> MPTQKELRDTMSKKLQEAIKHPDPAVVAGRKSAIKRWVGVLQDNFMEHIKYFKGDKLKFLHNVFQDEGCWSGVRLDNAALGQRFTEEKIGGIDNPLRKYEMACSYCVVDKIHPLFQKRFESYRNKFPPGAFDGKTETEFGKYVRNSLLDSIKRKGPVFDFWIDRESGELKKYDAVEGFDSAVKFKWSEGVEYFYNHLKEEDKEKKLTEAILALSRVQSVEKDAPILDFCVNKIVDKDTLLQKLSQKDKGVYSLFVELIESCFFDTVHDLVQCWCYKE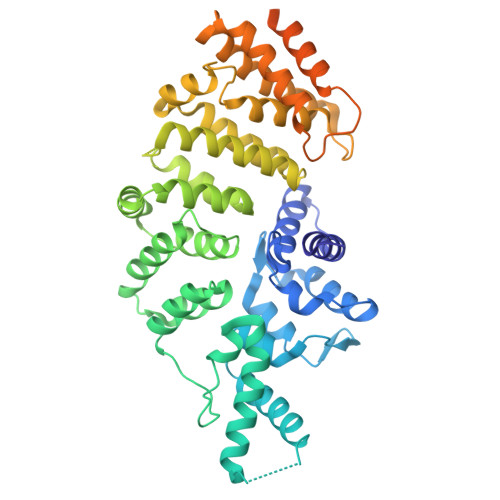VSAGGDHSEKIFSQRDYELFLSSLSDTMLKNPELSVQARSLIMEFWECGSLYQYRKAAVNTSNYTVPTSGVFAELIVNWRREDIYKTDEEKEIEKKEILDMMSFAKDCFPEKFELFKKLIIRDLRLCGREGKRVNVDYGLFAEELFSELEKTILPPGPVGDGPCSNLRSRSKAHGSKKTTLPVDDSPQSELGTPSVSGVSSYKKKSVFTLSGNKLEHHHHHH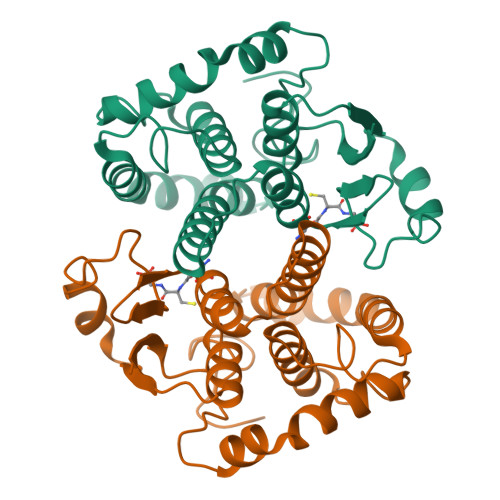>PAKLGYWKIRGLQQPVRLLLEYLGEKYEEQIYERDDGEKWFSKKFELGLDLPNLPYYIDDKCKLTQSLAILRYIADKHGMIGTTSEERARVSMIEGAAVDLRQGISRISYQPKFEQLKEGYLKDLPTTMKMWSDFLGKNPYLRGTSVSHVDFMVYEALDAIRYLEPHCLDHFPNLQQFMSRIEALPSIKAYMESNRFIKWPLNGWHAQFGGGDAPP[2x]> MGGKTVDQKTYSVGDTVKYTITYKNAVNYHGTEKVYQYVIKDTMPSASVVDLNEGSYEVTITDGSGNITTLTQGSEKATGKYNLLEENNNFTITIPWAATNTPTGNTQNGANDDFFYKGINTITVTYTGVLKSGAKPGSADLPENTNIATINPNTSNDDPGQ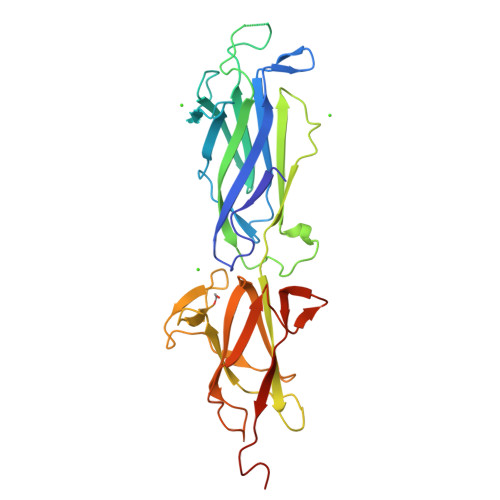KVTVRDGQITIKKIDGSTKASLQGAIFVLKNATGQFLNFNDTNNVEWGTEANATEYTTGADGIITITGLKEGTYYLVEKKAPLGYNLLDNSQKVILGDGATDTTNSDNLLVNPTVENNKGTELPSHHHHH N-{(1S,2R)-1-benzyl-2-hydroxy-3-[(1S)-1,2,3,4-tetrahydronaphthalen-1-ylamino]propyl}-3-(1,1-dioxido-1,2-thiazinan-2-yl)-5-(ethylamino)benzamide | 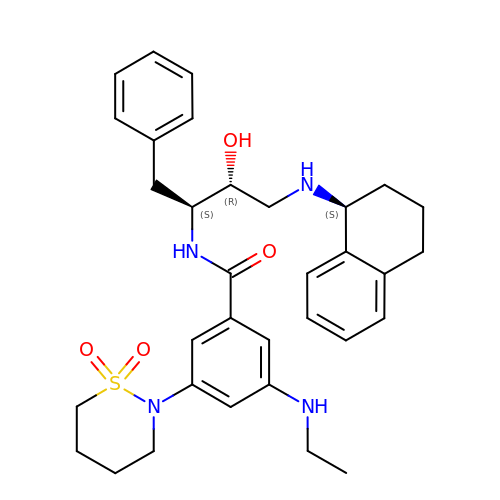C33 H42 N4 O4 S | OAOKRIOFVOASEG-OWHBQTKESA-N> GNNVVVLGTQWGDEGKGKIVDLLTERAKYVVRYQGGHNAGHTLVINGEKTVLHLIPSGILRENVTSIIGNGVVLSPAALMKEMKELEDRGIPVRERLLLSEACPLILDYHVALDNAREKARGAKAIGTTGRG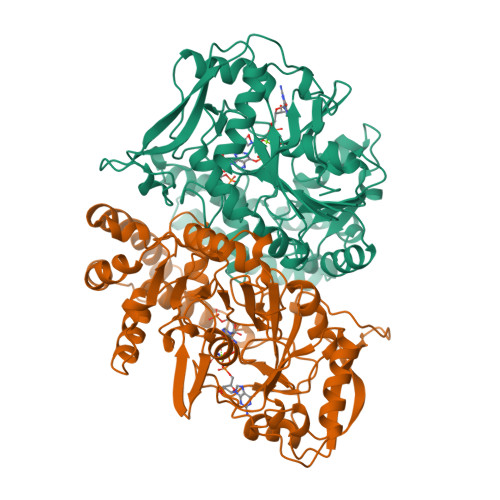IGPAYEDKVALRGLRVGDLFDKETFAEKLKEVMEYHNFQLVNYYKAEAVDYQKVLDDTMAVADILTSMVVDVSDLLDQARQRGDFVMFEGAQGTLLDIDHGTYPYVTSSNTTAGGVATGSGLGPRYVDYVLGILKAYSTRVGAGPFPTELFDETGEFLCKQGNEFGATTGRRRRTGWLDTVAVRRAVQLNSLSGFCLTKLDVLDGLKEVKLCVAYRMPDGREVTTTPLAADDWKGVEPIYETMPGWSESTFGVKDRSGLPQAALNYIKRIEELTGVPIDIISTGPDRTETMILRDPFDA>[2x]GPGSVPELKQISRVEAMRLGPGWSHS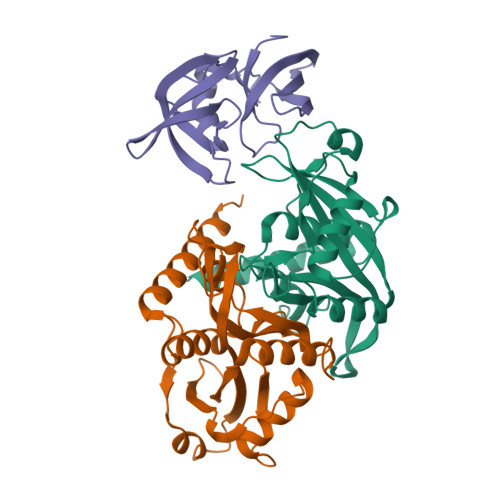CHAMLYAANPGQLFGRIPMRFSVLMQMRFDGLLGFPGGFVDRRFWSLEDGLNRVLGLGLGCLRLTEADYLSSHLTEGPHRVVAHLYARQLTLEQLHAVEISAVHSRDHGLEVLGLVRVPLYTQKDRVGGFPNFLSNAFVSTAKCQLLFALKVLNMMPEEKLVEALAAATEKQKKALEKLLPASS;> GPGSRSDSPEIPFQAAAGPSDGLDASSPGNSFVGLRVVAKWSSNGYFYSGKITRDVGAGKYKLLFDDGYECDVLGKDILLCDPIPLDTEVTALSEDEYFSAGVVKGHRKESGELYYSIEKEGQRKWYKRMAVILSLEQGNRLREQYGLGPYEAVTPLTKAADISLDNLVEGKRKRRSNVS> PP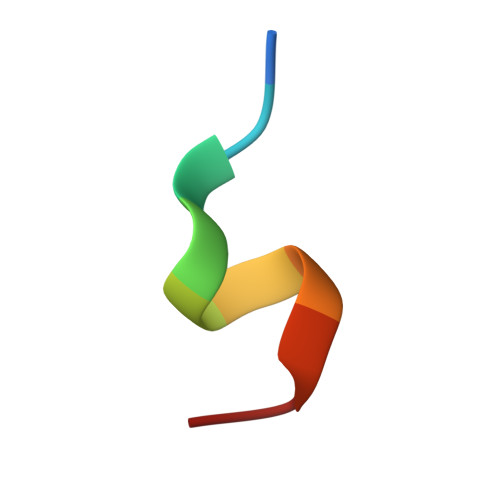TLHELYDL> EDVVWRWSCDNGKCVKLKNDPRSSEPALSLEACKMFCNEYGLLWPRPTGEADLGNFLSKINLNSIEVKILKKGATDDLMEAAAKRFKEQVSLAIPRGSTPKLTGKAVDVYLVNENPNEKAFSLEMDESYGLRVSPSGADRVNATITANSFFGMRHGLETLSQLFVFDDIR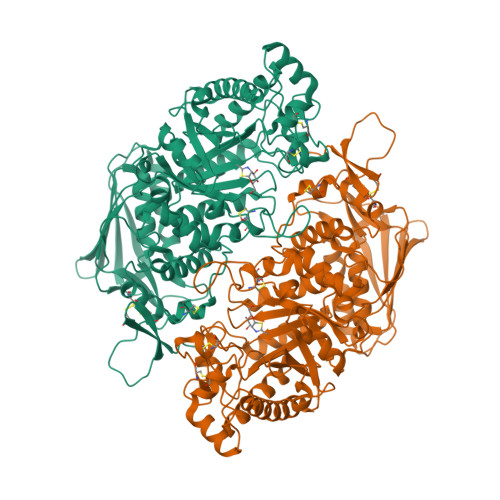DHLLMVRDVNISDKPVYPYRGILLDTARNYYSIESIKRTIEAMAAVKLNTFHWHITDSQSFPFVTTKRPNLYKFGALSPQKVYTKAAIREVVRFGLERGVRVLPEFDAPAHVGEGWQDTDLTVCFKAEPWKSYCVEPPCGQLNPTKDELYQYLEDIYSDMAEVFDTTDIFHMGGDEVSEACWNSSDSIQNFMMQNRWDLDKESFLKLWNYFQQKAQDKAYKAFGKKLPLILWTSTLTNYKHIDDYLNKDDYIIQVWTTGVDPQIKGLLEKGYRLIMSNYDALYFDCGYGAWVGAGNNWCSPYIGWQKVYDNSPAVIALEHRDQVLGGEAALWSEQSDTSTLDGRLWPRAAALAERLWAEPATSWQDAEYRMLHIRERLVRMGIQAESLQPEWCYQNEGYCYS> MKILVAVKQTAALEEDFEIREDGMDVDEDFMMYDLNEWD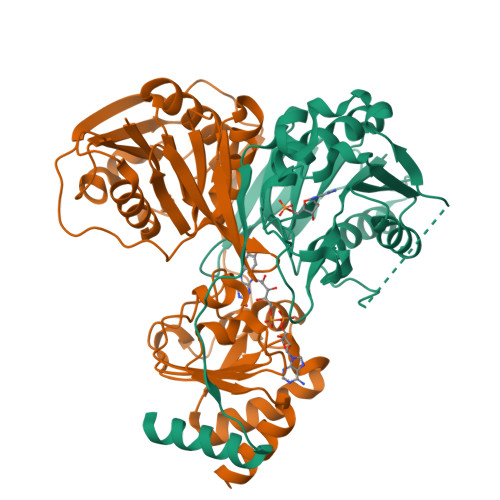DFSLEEAMKIKESSDTDVEVVVVSVGPDRVDESLRKCLAKGADRAVRVWDDAAEGSDAIVVGRILTEVIKKEAPDMVFAGVQSSDQAYASTGISVASYLNWPHAAVVADLQYKPGDNKAVIRRELEGGMLQEVEINCPAVLTIQLGINKPRYASLRGIKQAATKPIEEVSLADIGLSANDVGAAQSMSRVRRMYIPEKGRATMIEGTISEQAAKIIQIINEFKGA;> MSKILVIAEHRRNDLRPVSLELIGAANGLKKSGEDKVVVAVIGSQADAFVPALSVNGVDELVVVKGSSIDFDPDVFEASVSALIAAHNPSVVLLPHSVDSLGYASSLASKTGYGFATDVYIVEYQGDELVATRGGYNQKVNVEVDFPGKSTVVLTIRPSVFKPLEGAGSPVVSNVDAPSVQSRSQNKDYVEVGGGNDIDITTVDFIMSIGRGIGEETNVEQFRELADEAGATLCCSKPIADAGWLPKSRQVGQSGKVVGSCKLYVAMGISGSIQHMAGMKHVPTIIAVNTDPGASIFTIAKYGIVADIFDIEEELKAQLAA> HHHHHHSVFEDDLPFLEFTGSIVYSYDASDCSFLSEDISMSLSDGDVVGFDMEWPPLYNR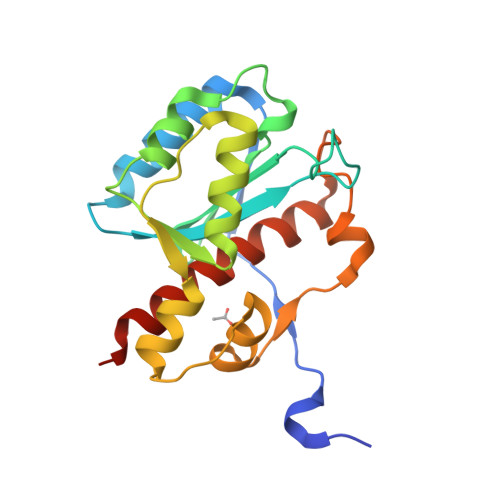GKLGKVALIQLCVSESKCYLFHVSSMSVFPQGLKMLLENKAVKKAGVGIEGDQWKLLRDFDIKLKNFVELTDVANKKLKCTETWSLNSLVKHLLGKQLLKDKSIRCSNWSKFPLTEDQKLYAATDAYAGFIIYRNLEILDDTVQR>AMAFYFEEPSRTFSEFLLVPGYSSAECVPTNVSLKTPIVKFKKGEESAITMNIPLVSAIMQAVSDDNMGIALATEGGVSFIFGSQSIESEAAMVSRVKNHKSGGRKDYDSNKENKLELLDSSKRYVVGAGINTRDYEERVPALVEAGADILCIDSSEGYSEWQKRTLDYVRGKYGDTVKVGAGNVVDRDGFRYLAEAGADFVKVGVGGGSICITREQKGIGRGQATALIDVAKARDEYFEETGVYIPICSDGGIVYDYHMTLALAMGADFIMLGRYFSRFDESPTNKVNLNGTYMKEYWGEGANRARNWQRYDLGGDKKLS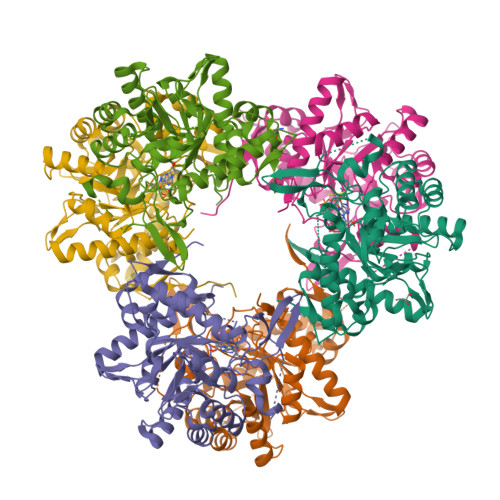FEEGVDSYVPYAGSLKDNVAISLSKVRSTMCNCGALNIPELQQKAKITLVSSTSIVEGGAHDVVVKDASNNLIK[6x]>[8x]YFQGMAKHAILVIDMLNDFVGEKAPLRCPGGETIIPDLQKIFEWVRGREGDDIHLVHIQEAHRKNDADFRVRPLHAVKGTWGSDFIPELYPQEDEYIVQKRRHSGF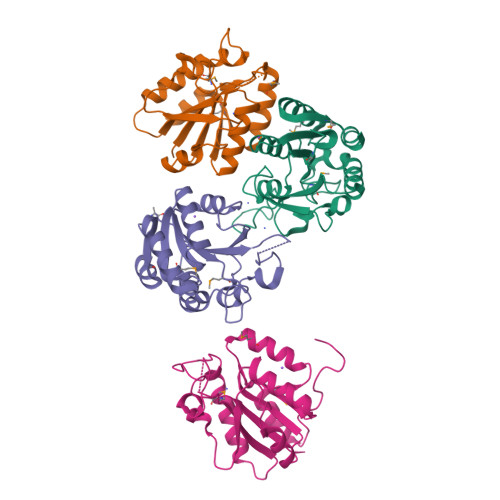AHTDLDLYLKEEGIDTVVLTGVWTNVCVRSTATDALANAYKVITLSDGTASKTEEMHEYGLNDLSIFTKVMTVDQYIQAWENDEDPWVGGGDAQNKVK>LRLPRETDEEPEEPGRRGSFVEMVDNLRGKSGQGYYVEMTVGSPPQTLNILVDTGSSNFAVGAAPHPFLHRYYQRQLSSTYRDLRKGVYVPYTQGKWEGELGTDLVSIPHGPNVTVRANIAAITESDKFFINGSNWEGILGLAYAEIARPDDSLEPFFDSLVKQTHVPNLFSLQLCGAGFPLNQSEVLASVGGSMIIGGIDHSLYTGSLWYTPIRREWYYEVIIVRVEINGQDLKMDCKEYNYDKSIVDSGTTNLRLPKKVFEAAVKSIKAASSTEKFPDGFWLGEQLVCWQAGTTPWNIFPVISLYLMGEVTNQSFRITILPQQYLRPVEDVATSQDDCYKFAISQSSTGTVMGAVIMEGFYVVFDRARKRIGFAV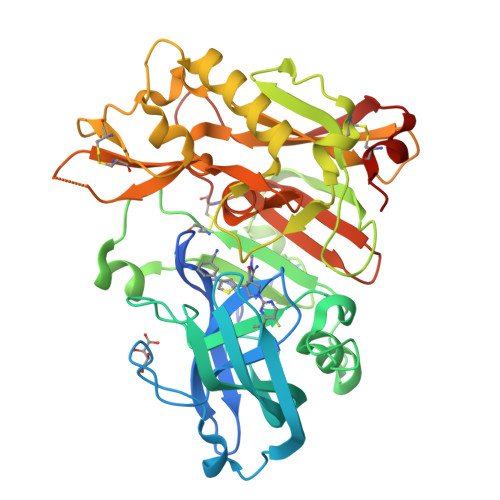SACHVHDEFRTAAVEGPFVTLDMEDCGYNIPQTDEST[2x]> INIQEDKLVSAHDAEEILRFFNCHDSALQQEATTLLTQEAHLLDIQAYRAWLEHCVGSEVQYQVISRELRAASERRYK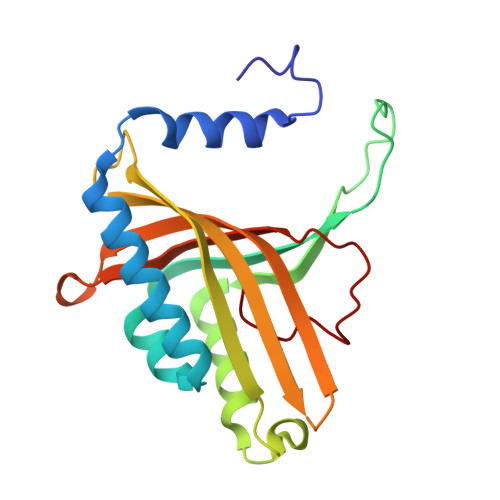LNEAMNVYNENFQQLKVRVEHQLDPQNWGNSPKLRFTRFITNVQAAMDVNDKELLHIRSNVILHRARRGNQVDVFYAAREDKWKRGEGGVRKLVQRFVDYPERILQTHNLMVFL> AGLCTSFKIVPIVPAQVPQDVLAYTFFTSSYAIQSPFPEAAVSRIVVHTRWASNVDFDRDSSVIMAPPTENNIHLFKQLLNTETLSVRGANPLMFRANVLHMLLEFVLDNLYLNRHTGFSQDHTPFTEGANLRSLPGPDAEKWYSIMYPTRMGTPNVSKICNFVASCVRNRVGRFDRAQMMNGAMSEWVDVFETSDALTVSIRGRWMARLARMNINPTEIEWALTECAQGYVTVTSPYAPSVNRLMPYRISNAERQISQIIRIMNIGNNATVIQPVLQDISVLLQRISPLQIDPTIISNTMSTLSPASSILGKLRPSNSDFSSFRVALAGWLYNGVVTTVIDDSSYPKDGGSVTSLENLWDFFILALALPLTTDPCAPVKAFMTLANMMVGFETIPMDNQIYTQSRRASAFSTPHTWPRCFMNIQLISPIDAPILRQWAEIIHRYWPNPSQIRYGAP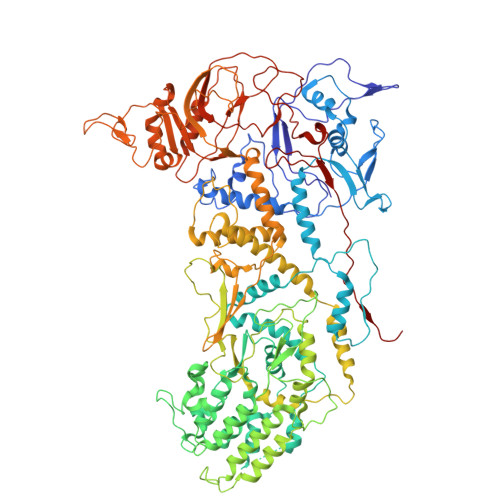NVFGSANLFTPPEVLLLPIDHQPANVTTPTLDFTNELTNWRARVCELMKNLVDNQRYQPGWTQSLVSSMRGTLDKLKLIKSMTPMYLQQLAPVELAVIAPMLPFPPFQVPYVRLDRDRVPTMVGVTRQSRDTITQPALSLSTTNTTVGVPLALDARAITVALLSGKYPPDLVTNVWYADAIYPMYADTEVFSNLQRDMITCEAVQTLVTLVAQISETQYPVDRYLDWIPSLRASAATAATFAEWVNTSMKTAFDLSDMLLEPLLSGDPRMTQLAIQYQQYNGRTFNVIPEMPGSVIADCVQLTAEVFNHEYNLFGIARGDIIIGRVQSTHLWSPLAPPPDLVFDRDTPGVHIFGRDCRISFGMNGAAPMIRDETGMMVPFEGNWIFPLALWQMNTRYFNQQFDAWIKTGELRIRIEMGAYPYMLHYYDPRQYANAWNLTSAWLEEITPTSIPSVPFMVPISSDHDISSAPAVQYIISTEYNDRSLFCTNSSSPQTIAGPDKHIPVERYNILTNPDAPPTQIQLPEVVDLYNVVTRYAYETPPITAVVMGVP> MAHHHHHHVDDDDKMVHHDGFQTVKATIDWEHPMFKLYEKAKRNGKWNPADIDFSQDQKDFASLTSEEKISALPLVAGFSAGEEAITLDILPMAHALARQGRLEDVLFLTTFMHDEAKHVEMFSRWQQAVGIGQMDLSVFHNDHYKRIFYEALPEAMNRLYADDSPEAVIRAATVYNMIVEGTLAESGYYTFRQIYKKAGLFPGLLQGIDYLNMDEGRHIQFGIYTIQRIVNEDERYYELFIRYMDELWPHVIGYVDYLTELGKRQQQLARTYALEIDYDLLRHYVIKQFNLRKKQISRTKRVDVVEGLEKTAAES

The heterodinuclear Mn/Fe cofactor is found in the R2 subunits of subclass Ic ribonucleotide reductases (denoted as R2c) as well as a related group of proteins known as R2-like ligand-binding oxidases (R2lox). Although the physiological function of R2lox proteins is not known, the cofactor catalyzes formation of a tyrosine–valine ether cross-link in the protein scaffold. Two proteins from this group have been characterized to date, homologs from Mycobacterium tuberculosis and Geobacillus kaustophilus. Both contain the ether cross-link, and both co-purify from heterologous expression hosts with a long-chain fatty acid ligand bound in a hydrophobic channel leading from the protein surface to the active site, hence the name ligand-binding oxidase. The two metal ions are bound next to each other in octahedral geometry by two histidines and four glutamates, with the manganese ion occupying the N-terminal metal-binding site 1.

Crystal structures were obtained of all three R2lox point mutants in the non-activated reduced and the oxidized resting state by soaking apo-protein crystals with MnII and FeII under anoxic or aerobic conditions, respectively. In contrast, the bulky isoleucine side chain in V72I-R2lox has a larger effect on Y162 than on the metal-coordinating residues. It seems to have displaced the Y162 side chain, particularly in the reduced state. Both I72 and Y162 were difficult to place in the electron density. Aside from these two residues, however, the structures of V72I-R2lox are practically identical to the wild-type structures in both redox states. Interestingly, it appears as if the ether cross-link was formed between the hydroxyl group of Y162 and the Cβ of I72 in the oxidized state. Although the model with an ether linkage is more convincing than other models with different rotamers of the two residues, because the electron density is ambiguous, we used mass spectrometry to verify if the cross-link is present. More mass spectrometry samples were consequently prepared in the dark. The Y162-I72 cross-linked peptide was obtained by digestion of aerobically Mn/Fe-reconstituted V72I-R2lox, but only if the samples were processed in the dark, whereas the cross-link was not present in V72L-R2lox (Fig. S1 and data not shown). Therefore, an isoleucine in position 72 allows cross-link formation, but makes the link more susceptible to destruction by photoactivation.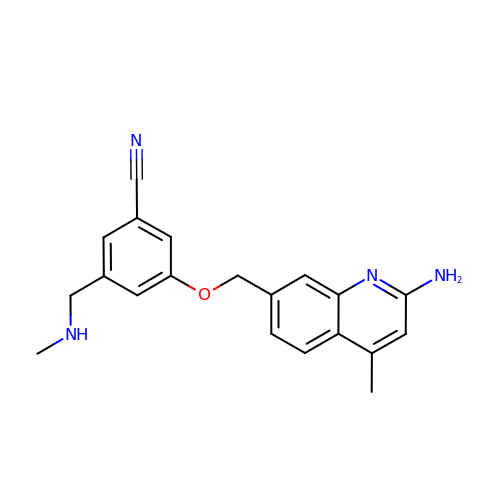3-[(2-amino-4-methylquinolin-7-yl)methoxy]-5-[(methylamino)methyl]benzonitrile | C20 H20 N4 O | NLOWGCVMDAJXMN-UHFFFAOYSA-N>MSRVLLCSAGHSSMVVPEAFHAVPEGFEEVHVFTTDSEKFNPVVLNDFFHSLPNVRFSITKCHGLADILNERDFEFYQEMLWQWYLTKMPDNELPYVCLSGGIKSMSASLQKAATLFGAQSVFHVLADNNPRNIEEMFDALQKGQIHFIEMGYEPGWAALRRLKKI[4x]

In order to identify novel CARF effectors, we used Foldseek18 to search for proteins with structural homology to CARF domain of the Cam1 effector. This method rendered a 600-residue protein containing an N-terminal CARF domain followed by a linker region and a C-terminal adenosine deaminase (ADA) domain, with accession number HAJ98955.1 from an unknown Bacteriodales bacterium (hereafter named CRISPR-associated deaminase, CRISPR-associated adenosine deaminase 1 [Cad1]), for which homologs were already identified in a previous bioinformatic screen. cad1 is located immediately downstream the cas10-csm genes of a type III-A CRISPR locus. Further analysis of cad1 homologs showed that over 70% associate in genomes containing type III systems (mostly belonging to the A and B subtypes) and exist within many unique phyla of bacteria. These data suggest that Cad1 is a widespread effector in type III CRISPR-Cas systems. Altogether, these data demonstrate that Cad1 deaminates ATP molecules to ITP through the formation of an hexameric complex that requires a Mg+2 or Mn+2 cofactor and an activating cA4 or cA6 ligand. While the triggering of a growth arrest in the host is a common strategy of all CARF effectors, we believe that Cad1 introduces a new mode of defense for CRISPR-Cas systems that couples nucleotide deamination activity to a sequence-specific, RNA-guided adaptive immune response.

Next, we used X-ray crystallography to elucidate the molecular details of cOA interactions with Cad1’s CARF domain. We first solved the crystal structure of apo-Cad1-CARF-His6 at 3.6 Å resolution. The structure showed an asymmetric unit composed of a tetramer formed by crystal packing between two Cad1-CARF-His6 dimers in which monomers are arranged in a pseudo-2-fold symmetry. Consistent with these results, SECMALS analysis of Cad1-CARF-His6 showed the formation a stable dimer in solution. Analysis of the electrostatic potential revealed the presence of a positively charged pocket that harbors both K104 residues on top of the C-terminal legs (residues 104–117) on each of the CARF monomers at the dimeric interface. Although both cOA ligands were fully accommodated in the electropositive pocket of apo Cad1-CARF-His6, they affected differently the angle between the two C-terminal legs of the CARF monomers. While cA6 binding produced a minor change (from 58° in the apo structure to 55°), cA4 binding opened this angle to 76°, most likely a consequence of the deep burial of cA4 within the pocket.>MTMDEQQSQAVAPVYVGGFLARYDQSPDEARLLLPRDVVEHWLHAQGQGQPSLSVALPLNINHDDTAVVGHVAAMQSVRDGLFCLGCVTSPRFLEIVRRASEKSELVSRGPVSPLQPDKV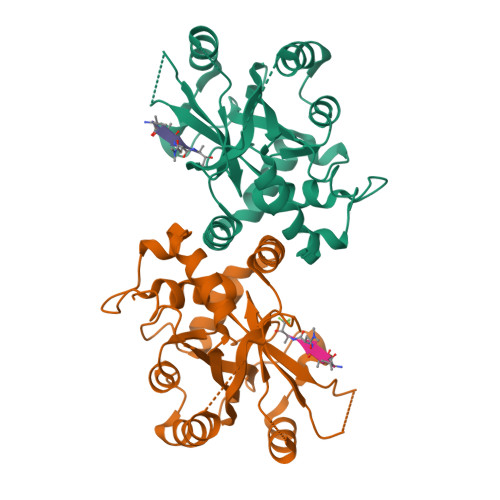VEFLSGSYAGLSLSSRRCDDVEQATSLSGSETTPFKHVALCSVGRRRGTLAVYGRDPEWVTQRFPDLTAADRDGLRAQWQRCGSTAVDASGDPFRSDSYGLLGNSVDALYIRERLPKLRYDKQLVGVTERESYVKA[4x]Rhodotorula dairenensis β-fructofuranosidase is a highly glycosylated enzyme with broad substrate specificity that catalyzes the synthesis of 6-kestose and a mixture of the three series of fructooligosaccharides (FOS), fructosylating a variety of carbohydrates and other molecules as alditols. RdINV subunit is composed of two domains, similar to the rest of the reported fungal β-fructofuranosidases within GH32. The β-propeller catalytic domain contains residues 185 to 487 and is constituted by five blades (I-V), each involving four antiparallel β-strands (ABCD) with a “W” topology. The β-sandwich domain, extending from residue 495 to 673, is composed of twelve β-sheets ordered in two six-stranded clusters of antiparallel β-strands.

To analyze its hydrolytic activity, the inactivated D188A-RdINVΔ21–139 mutant was deglycosylated, crystallized and used for soaking experiments with different sugars, including fructose, sucrose, 1-kestose, raffinose or nystose, and, also, ternary complexes with fructose and palatinose, trehalose or hydroxytyrosol have also been pursued. However, only complexes of this truncated variant with fructose, sucrose or raffinose were obtained, the crystals belonging to the P21 space group with two complete dimers within the asymmetric unit that are essentially similar. To obtain the D188A-RdINVΔ21–139 raffinose complex, a crystal grown in 20% PEG 3350, 0.2 M NaCl, 0.1 M Bis-Tris pH 5.5 (2:1 rate) was transferred for 2 h to a soaking solution containing mother liquor supplemented with 30 mM raffinose. Diffraction data of D188A-RdINVΔ21–139 in complex with fructose, sucrose and raffinose were collected at the ALBA synchrotron station (Barcelona, Spain), being indexed in the P21 space group with four molecules in the asymmetric unit, at 1.86 Å, 2.38 Å and 2.27 Å, respectively. On the other hand, the sucrose and the raffinose complexes are essentially identical in the common portion, an issue that may explain that the specific hydrolytic activity observed on this three-saccharide is very similar to that reported on sucrose hydrolysis. Therefore, the description of subsites +1 and +2 will be based on the complex with raffinose. The glucose bound at subsite +1 is tightly fixed by direct hydrogen bonds to the acid/base catalytic Glu362 (through its O2), and to Asn387 (O2 and O3), with additional water-mediated links from both residues to O3. Similarly, O4 is linked to Gln280 and Arg311 through a water molecule that also makes a polar link to the O6 oxygen from galactose located at +2 subsite. This O6 participates in a well-ordered net of water molecules linking the substrate to Asn275, Gln280 and Asn308, with Asn275 being also water-linked to the galactose O4 and O5 atoms.

>MKFTLLSVVAIAAAASDSYAAPAASSLAGPVTTGVFSAVSAIPSFATNLSGQVASATSTVLSGSTASGSSATAAPSASASGASSMQSMASSLSGSAFSPSSMMPIASGNMTMPNMTSSASASSAASTATGVAGGAGSNSSSSCAPTSLPASATELPTTVPTGTVITGDYTGSYRPQVHYSPPKGFMNAPNGCHRDRNGTYHLYYQYNPLEYVAGNQHWGHATSDDLYHWTNQPIAIFPPNSTSQVFSGSAVLDPNNTSGFFPNTTDGVVAVYTLNTPTLQVQEVAYSTDGGYNFTPYENNPVLSVGSNQFRDPKVFWYEDHWVMAVAAANDFTIEIYTSPNLTSWTFASNFTHHGLLGLAYECPNLVQVPFQDDPSKSAWLMYISINPGAPLGGSVGQYFPGDFNGTHFVAYDSAARIADFAKDNYASQWFADTENGESISIAWASNWQYTQQVPTSAQAFRSAMSLPRRNYLTNITRLGWDLVSLPYDLSPVVGPSLLSSSEANSTADVDFTNVTSNAVWFSLNVTLPDAAIQNASLISADASINITFLPSTKCSSSSGSGSDSPAATLTYFYAGLTNGALALTRPAASSSWGAENPFFTDKFSYTLVDPLTSLVGVFDRSMLEVFVNEGAHSATMLVFPDSPVGSMKVATGGLPEGTQVNLQVNGLESTWQSS[4x]>AYLLFYTEAK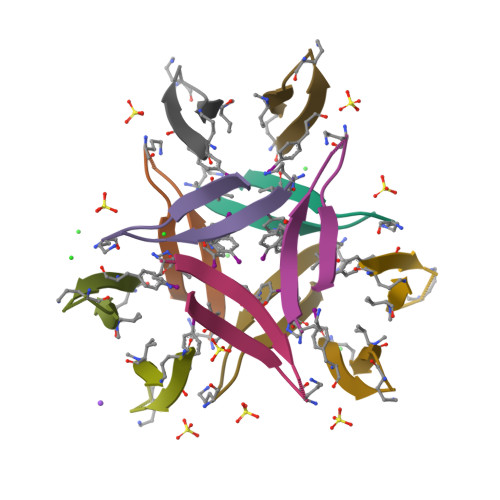VAVAVK[12x]> XYRIPSYDFADEA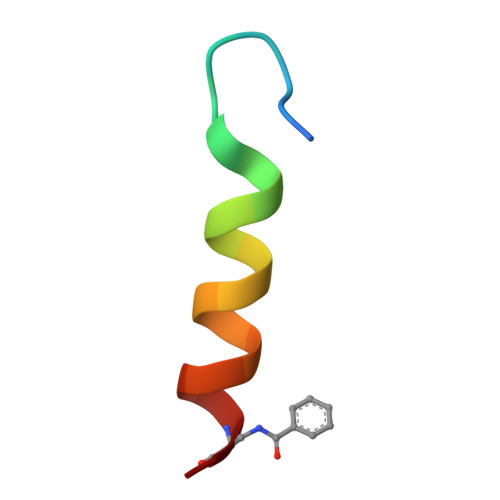EKLLRDAAG>[3x]MATNFFIQPITEEAEAYYPPSVITNKRKDLGVDVYCCSDLVLQPGLNIVRLHIKVACEHMGKKCGFKIMARSSMCTHERLLILANGIGLIDPGYVGELMLKIINLGDTPVQIWAKECLVQLVAQGDHVPDHINILKRNQIFPLFAPTPRGEGRFGSTGEAGIMRT

Deoxyuridine 5'-triphosphate nucleotidohydrolase (dUTPase, EC 3.6.1.23) is a ubiquitous enzyme in DNA repair that plays a key role in preventing uracil from being incorporated into DNA. dUTPases are widespread in organisms, including eukaryotes, prokaryotes, and some viruses. On the one hand, it catalyzes the cleavage of dUTP into dUMP and pyrophosphate (PPi), which reduces the possibility that dUTP will be incorporated into DNA through DNA polymerase. Herein, we determine the crystal structures of ASFV dUTPase and swine dUTPase in both their ligand-free and ligand-bound forms. We observe that the swine enzyme employs a classical dUTPase architecture made up of three-subunit active sites, whereas the ASFV enzyme employs a novel two-subunit active site.

The α,β-bridging oxygen in dUTP was replaced by an imido group to form 2′-deoxyuridine 5′-(α,β-imido) triphosphate (dUPNPP), a nonhydrolyzable substrate analog and potent competitive inhibitor of dUTPase. The aDUT-dUPNPP-Mg2+ complex structure represents the prereaction state of the substrates just after binding to the active site. The crystal of the aDUT-dUPNPP-Mg2+ complex grew in the P212121 space group with one trimer in each asymmetric unit. Fortunately, clear electron density was observed for the remaining C-terminal residues in the aDUT-dUPNPP-Mg2+ complex structure. However, surprisingly, there is no C-terminal β-strand swapping in ASFV dUTPase, and the aDUT-dUPNPP-Mg2+ structure provides definite evidence to support the presence of two-subunit active sites in the trimeric dUTPase. The ASFV dUTPase active site is formed by the following two subunits: one subunit provides catalytic motifs I, II, and IV and the other subunit provides motifs III and V. The C terminus (motif V) of ASFV dUTPase continues to reach the active site of its own subunit instead of reaching the third subunit as seen in a classical dUTPase. When dUTP and Mg2+ enter the active site pocket, the uracil ring forms hydrogen bonds with the main-chain oxygen and nitrogen of Met99, and the resultant hydrogen bonds can recognize and fix the uracil ring by imitating Watson–Crick pairing. The C terminus (motif V) changes to a closed state, closing the active site. Phe154 is conjugated with uracil to further fix the uracil ring.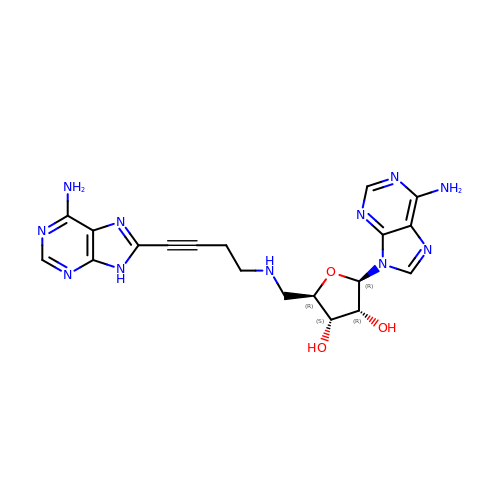(2~{R},3~{R},4~{S},5~{R})-2-(6-aminopurin-9-yl)-5-[[4-(6-azanyl-9~{H}-purin-8-yl)but-3-ynylamino]methyl]oxolane-3,4-diol | C19 H21 N11 O3 | ZVZLLIKFDIWTQZ-NBKUUXFISA-N> MPENVAPRSGATAGAAGGRGKGAYQDRDKPAQIRFSNISAAKAVADAIRTSLGPKGMDKMIQDGKGDVTITNDGATILKQMQVLHPAARMLVELSKAQDIEAGDGTTSVVIIAGSLLDSCTKLLQKGIHPTIISESFQKALEKGIEILTDM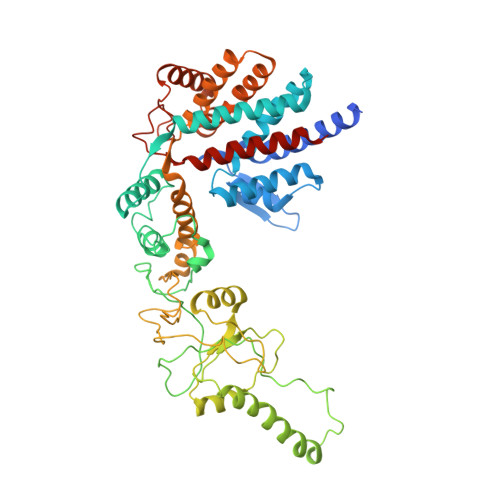SRPVELSDRETLLNSATTSLNSKVVSQYSSLLSPMSVNAVMKVIDPATATSVDLRDIKIVKKLGGTIDDCELVEGLVLTQKVSNSGITRVEKAKIGLIQFCLSAPKTDMDNQIVVSDYAQMDRVLREERAYILNLVKQIKKTGCNVLLIQKSILRDALSDLALHFLNKMKIMVIKDIEREDIEFICKTIGTKPVAHIDQFTADMLGSAELAEEVNLNGSGKLLKITGCASPGKTVTIVVRGSNKLVIEEAERSIHDALCVIRCLVKKRALIAGGGAPEIELALRLTEYSRTLSGMESYCVRAFADAMEVIPSTLAENAGLNPISTVTELRNRHAQGEKTAGINVRKGGISNILEELVVQPLLVSVSALTLATETVRSILKIDDVVNTR>APAFSVSPASGLSDGQSVSVSVSGAAAGETYYIAQCAPVGGQ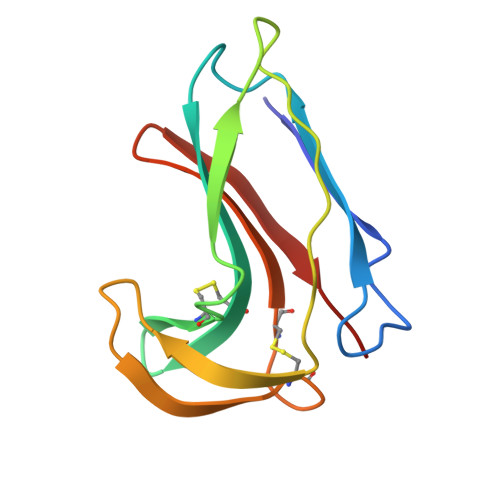DACNPATATSFTTDASGAASFSFVVRKSYTGSTPEGTPVGSVDCATAACNLGAGNSGLDLGHVALTFG[2x]2-AMINO-5-BROMO-6-PHENYLPYRIMIDIN-4-OL | C10 H8 Br N3 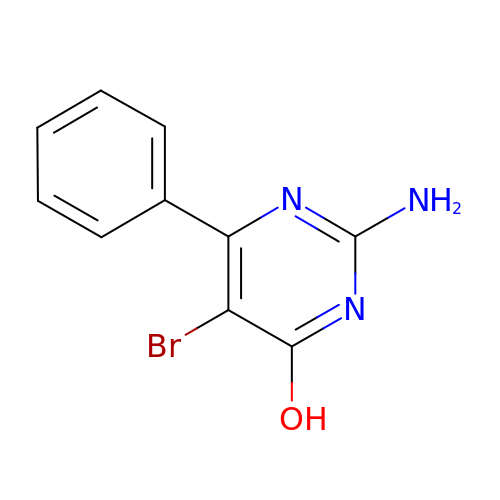O | CIUUIPMOFZIWIZ-UHFFFAOYSA-N>GSHMTADKHEVLLRMRAIELLAYWEGRLVTTRLMNWFGLSRQQASADIKRYNTLYNPDALIHDPSVKGYVPKASFQPVLTTAHINEYLNMLSGLVSESHALIAMPEPNLAAVQLPDRSVRPEVIREVLRACRNQSTLKMIYASMQNPQWHERIISPHTLVYTGFRWHVRAYCHQSKQFKDFLLSRIDRTPVVVAIESVDPAQDQQWHEEIVLTLIPNPKLNSSQQALVEKDFGMPDGRLQIPVKKALAHYTLQRYQTAITLAEAEDALKYPLVLQRSDIEKLSSYLFDQAS[2x]

Bacteriophage exclusion (‘BREX’) phage restriction systems are found in a wide range of bacteria. Biochemical and crystallographic analyses of this factor, which we term BrxR (‘BREX Regulator’), demonstrate that it forms a homodimer and specifically binds a DNA target site upstream of its transcription start site. We demonstrate that BrxR is a sequence-specific DNA binding protein comprising wHTH, WYL and WCX domains, propose that the protein and its reading frame act respectively as trans and cis transcriptional regulators of the BREX system, and suggest that its function has been widely adopted in more divergent bacterial species to regulate defense systems. Bioinformatic analyses indicated that BrxR contains three domains: an N-terminal winged helix-turn-helix (wHTH) domain, a WYL domain and a ‘WYL C-terminal extension’ (‘WCX’) domain.

We next co-crystallized BrxR with this palindromic sequence and solved a second structure of BrxR bound to the DNA target at 2.3 Å resolution. The cocrystal structure illustrates that BrxR binds the DNA target through extensive interactions between each subunit's wHTH domain and each corresponding target half-site. The DNA duplex maintains a B-form topology and all the bases are found in Watson-Crick interactions with their partners from the opposing complementary strand. The DNA is bent by ∼10–15° within the plane of the protein–DNA complex, and the minor groove is significantly narrowed across the central five base pair sequence that separates the two related target half-sites. Overlay of the DNA-bound protein structure to the unbound form of BrxR shows a near perfect match in structure, indicating that the unbound form of BrxR is in the proper configuration for binding this sequence. Each protein subunit contributes an interface that buries ∼870 Å2 of surface area, via the formation direct and water-mediated atomic contacts to the DNA (analysis facilitated and visualized with the DNAProDB online tool). BrxR makes relatively few direct contacts to bases in each half-site of the DNA target. One residue in particular (R38) appears to be involved in direct recognition of two consecutive bases in each half-site (G:C and T:A at positions ±6 and 7). K64 also appears to make multiple direct contacts, albeit in the minor groove, contacting bases at position ±10 and 11. Beyond these direct contacts, the substantial bend in the DNA target likely contributes to specificity across the center of the target, by promoting the A:T rich sequence across those basepairs.>KHSLPDLPYDYGALEPHINAQIMQLHHSKHHAAVVNNLNVTEEKYQEALAKGDVTAQIALQPALKFNGGGHINHSIFWTNLSPNGGGEPKGELLEAIKRDFGSFDKFKEKLTAASVGVQGSGWGWLGFNKERGHLQIAACPNQDPLQGTTGLIPLLGIDVWEHAYYLQYKNVRPDYLKAIW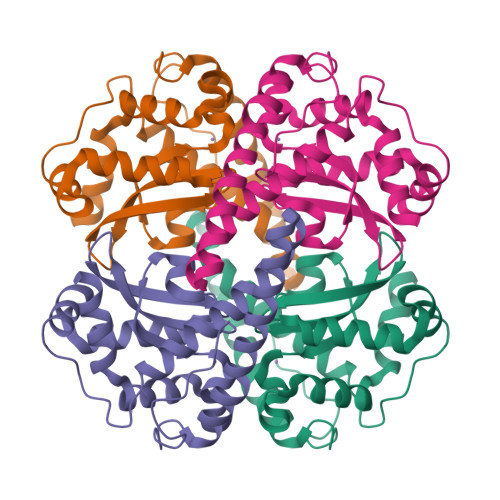NVINWENVTERYMACKK[2x]BMP9, a member of the TGFβ superfamily, is a homodimer that forms a signaling complex with two type I and two type II receptors. Signaling through high-affinity activin receptor-like kinase 1 (ALK1) in endothelial cells, circulating BMP9 acts as a vascular quiescence factor, maintaining endothelial homeostasis. BMP9 is produced by hepatocytes as the prepro-form and is processed by proprotein convertase in the trans-Golgi network into prodomain and mature BMP9 ligand. The endothelial ALK1/BMPR-II pathway is constitutively activated by circulating BMP9, the only confirmed BMP that circulates at active concentrations.

Here, we showed by chromatography and a 1.9 Å crystal structure that stable BMP9 dimers could form either with (D-form) or without (M-form) an intermolecular disulfide bond. A single crystal contained both D- and M-forms of HBMP9. Because two previously published BMP9 structures were either in the M-form or the D-form and crystallized under different protein-protein interaction contexts, our crystal is unique in addressing the local differences between D- and M-forms of BMP9 under identical conditions. We solved the structure to 1.9 Å with a space group I4122. Indeed, Cys-73, the critical amino acid involved in disulfide bond formation, was in two conformations as demonstrated by clear electron density, with an intermolecular disulfide bond formed between the two monomers in one of the conformations. Interestingly, no other major difference could be observed for the remaining residues between the D- and M-forms. Overlaying the HBMP9 structure with the previously published BMP9 structures revealed that the core regions of BMP9 were almost identical. Loops contacting the type I and type II receptors had diverged conformations. These are also the regions with the highest B factors in all BMP9 structures, indicating an intrinsically higher degree of flexibility at these regions.

> SHHHHHHAGAGSHCQKTSLRVNFEDIGWDSWIIAPKEYEAYECKGGCFFPLADDVTPTKHAIVQTLVHLKFPTKVGKACCVPTKLSPISVLYKDDMGVPTLKYHYEGMSVAECGCR> GTTEGDEEDATEAWRLHQKHVFVLSEAGKPVYSRYGSEEALSSTMGVMVALVSFLEADKNAIRSIHADGYKVVFVRRSPLVLVAVARTRQSAQELAQELLYIYYQILSLLTGAQLSHIFQQKQNYDLRRLLSGSERITDNLLQLMARDPSFLMGAARCLPLAAAVRDTVSASLQQARARSLVFSILLARNQLVALVRRKDQFLHPIDLHLLFNLISSSSSFREGEAWTPVCLPKFNAAGFFHAHISYLEPDTDLCLLLVSTDREDFFAVSDCRRRFQERLRKRGAHLALREALRTPYYSVAQVGIPDLRHFLYKSKSSGLFTSPEIEAPYTSEEEQERLLGLYQYLHSRAHNASRPLKTIYYTGPNENLLAWVTGAFELYMCYSPLGTKASAVSAIHKLMRWIRKEEDRLFILTPLTY;> MAAAAAGAGSGPWAAQEKQFPPALLSFFIYNPRFGPREGQEENKILFYHPNEVEKNEKIRNVGLCEAIVQFTRTFSPSKPAKSLHTQKNRQFFNEPEENFWMVMVVRNPIIEKQSKDGKPVIEYQEEELLDKVYSSVLRQCYSMYKLFNGTFLKAMEDGGVKLLKERLEKFFHRYLQTLHLQSCDLLDIFGGISFFPLDKMTYLKIQSFINRMEESLNIVKYTAFLYNDQLIWSGLEQDDMRILYKYLTTSLFPRHIEPELAGRDSPIRAEMPGNLQHYGRFLTGPLNLNDPDAKCRFPKIFVNTDDTYEELHLIVYKAMSAAVCFMIDASVHPTLDFCRRLDSIVGPQLTVLASDICEQFNINKRMSGSEKEPQFKFIYFNHMNLAEKSTVHMRKTPSVSLTSVHPDLMKILGDINSDFTRVDEDEEIIVKAMSDYWVVGKKSDRRELYVILNQKNANLIEVNEEVKKLCATQFNNIFFLD;> MGEEDYYLELCERPVQFEKANPVNCVFFDEANKQVFAVRSGGATGVVVKGPDDRNPISFRMDDKGEVKCIKFSLENKILAVQRTSKTVDFCNFIPDNSQLEYTQECKTKNANILGFCWTSSTEIVFITDQGIEFYQVLPEKRSLKLLKSHNLNVNWYMYCPESAVILLSTTVLENVLQPFHFRAGTMSKLPKFEIELPAAPKSTKPSLSERDIAMATIYGQLYVLFLRHHSRTSNSTGAEVVLYHLPREGACKKMHILKLNRTGKFALNVVDNLVVVHHQDTETSVIFDIKLRGEFDGSVTFHHPVLPARSIQPYQIPITGPAAVTSQSPVPCKLYSSSWIVFQPDIIISASQGYLWNLQVKLEPIVNLLPDKGRLMDFLLQRKECKMVILSVCSQMLSESDRASLPVIATVFDKLNHEYKKYLDAEQSYAMAVEAGQSRSSPLLKRPVRTQAVLDQSDVYTHVLSAFVEKKEMPHKFVIAVLMEYIRSLNQFQIAVQHYLHELVIKTLVQHNLFYMLHQFLQYHVLSDSKPLACL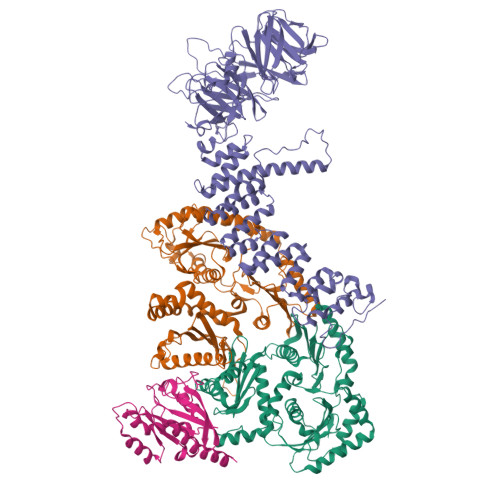LLSLESFYPPAHQLSLDMLKRLSTANDEIVEVLLSKHQVLAALRFIRGIGGHDNISARKFLDAAKQTEDNMLFYTIFRFFEQRNQRLRGSPNFTPGEHCEEHVAFFKQIFGDQALMRPTTF;> MTSRKKVLLKVIILGDSGVGKNSLMNQYVNKKFSNQYKATIGADFLTKEVMVDDRLVTMQIWDTAGQERFQSLGVAFYRGADCCVLVFDVTAPNTFKTLDSWRDEFLIQASPRDPENFPFVVLGNKIDLENRQVATKRAQAWCYSKNNIPYFETSAKEAINVEQAFQTIARNALKQETEVELYNEFPEPIKLDKNDRAKASAESCSC> GPLGS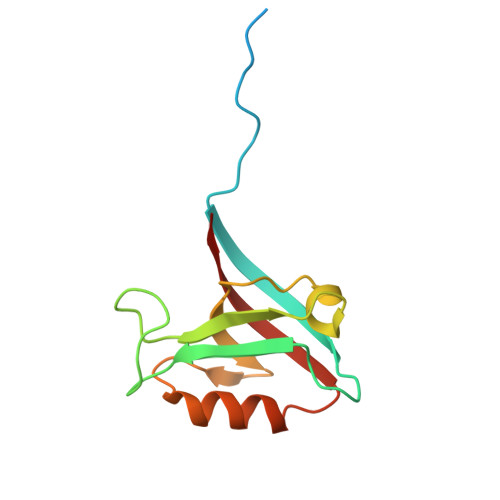SAPSVKGVSFDQANNLLIEPARIEEEELTLTILRQTGGLGISIAGGKGSTPYKGDDEGIFISRVSEEGPAARAGVRVGDKLLEVNGVALQGAEHHEAVEALRGAGTAVQMRVWRERM> MGVAQNNVDMEEGTLEVAMEYRTVT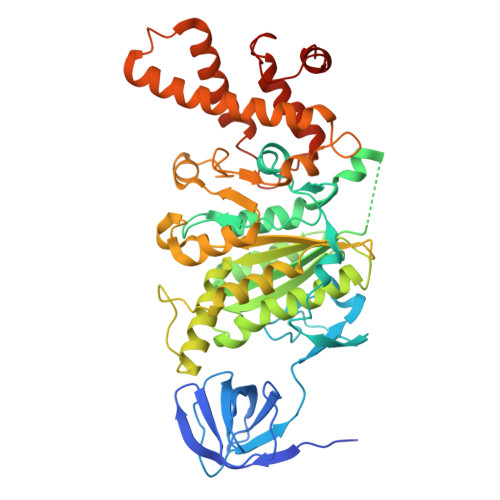GVAGPLVILDKVKGPKYYEIVNIRLGDGTMRRGQVLEVDGEKAVVQVFEGTSGIDNKFTTVQFTGEVLKTPVSLDMLGRIFNGSGKPIDNGPPILPEAYLDISGSSINPSERTYPEEMIQTGISTIDVMNSIARGQKIPLFSAAGLPHNEIAAQICRQAGLVKRLEKTDNLLEDGEEDNFAIVFAAMGVNMETAQFFKRDFEENGSMERVTLFLNLANDPTIERIITPRIALTTAEYLAYECGKHVLVILTDMSSYADALREVSAAREEVPGRRGYPGYMYTDLAQIYERAGRIEGRKGSITQIPILTMPNDDITHPTPDLTGYITEGQIYIDRQLQNRQIYPPINVLPSLSRLMKSAIGEGMTRRDHSDVSNQLYANYAIGKDVQAMKAVVGEEALSSEDLLYLEFLDKFERKFVAQGAYDSRNIFQSLDLAWTLLRIFPRELLHRIPGKTLDQYYSRDAAN oxidanyl dihydrogen phosphate | H3 O5 P | 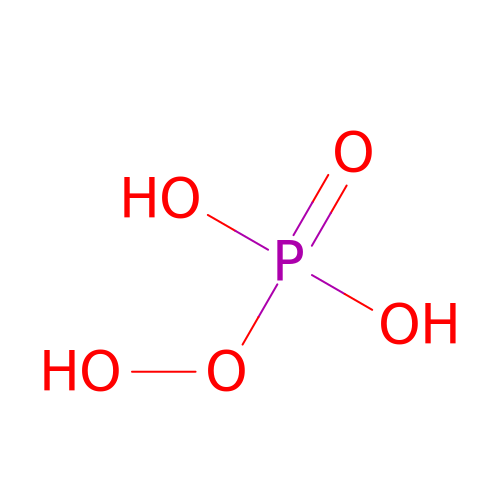MPNNOLHYOHFJKL-UHFFFAOYSA-N> MAPALVAAFGGKENITNLDACITRLRVSVADVSKVDQAGLKKLGAAGVVVAG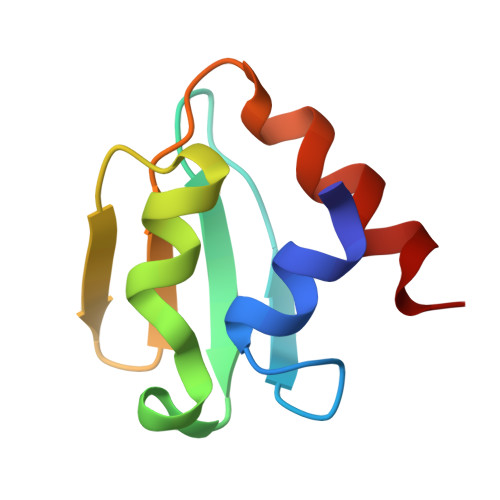SGVQAIFGTKSDNLKTEMDEYIR(2R)-2-{[6-(4-aminopiperidin-1-yl)-3,5-dicyano-4-ethylpyridin-2-yl]amino}-2-phenylacetamide | C22 H25 N7 O | 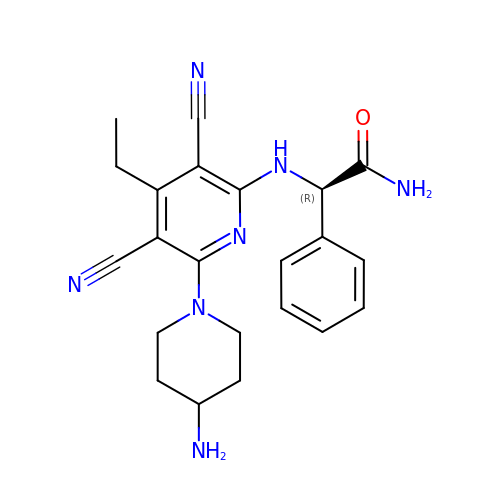KTLVWLAGCPGLOU-LJQANCHMSA-N> MNSQYMFDYPAINIDVRCHRLLSSVSYVAYNKFHTHDVSTYEHCEIPLEKLRLGFGRRNSLADFYSLGELPASWGPACYFSSVKPMMYTFQGMASDLSRF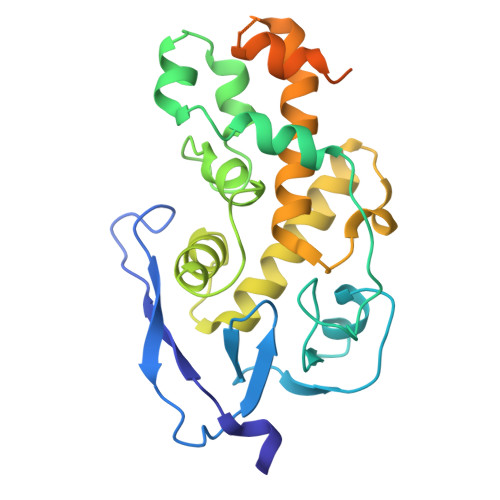DLTSFSRKGLPNVLKALSWPLGIPDCEIFSICSDRFVRGLQTRDQLMSYILRMGDSHSLDECIVQAHKKILQEARRLGLSDEHYNGYDLFREIGSLVCLRLINAEPFDTASSGEALDVRTVIRSYRASDPSTGLTEYGNSLWTPIHSHVDENDESSSDSDFGSHHHHHH>MKFPHDFLFGAASASYQVEGAWNEDGKGVTNWDEFSKIPGKTYNGTNGDIAVDHYHRYKEDVRLMAEMGLESYRFSISWARILPTGDGKVNEKGIEFYNNLIDECLKYGIVPFVTLYHWDLPLPLEKDGGWTNKRTAEAFVKYAETCFKAFGDRVKHWITFNETVMFCGLGYLKGAHPPGIQNDVPKYFQATHYVFYAHAKTVAVYKQLKQYGEIGITHVFLPAYSVDDQKENIQAANHANEYETYWYYDPILKGEYPSYVVQQLKEKGWTPNWTVEELEIIKQNAEENDFIGLNYYQPIRVERYDMDIKSEEHSRENSTLAPGNPSFDGFYRTVKMDDKTYTKWGWEISPEGFLEGLHMLKARYGDIKMYVTENGLGDEDPIIDGEIVDVPRIKFIEAHLKVMKRAIEEGINLKGYYAWSVIDLLSWLNGYKKQYGFIFVDHNDNLKRKKKLSFHWYKRVVETRGEELHHHHHH[2x]

In summary, we have characterized a novel PvGal-ase encoded by ORF1119 in Bacillus strain HMA207. The overall structure of ORF1119 was similar to those of other GH1 enzymes, which have a typical (β/α)8 barrel fold. The active site is located at the bottom of the pocket formed by loops of the barrel, a characteristic of most GH1 enzymes. The catalytic nucleophile (E374) and the catalytic acid/base (E163) residues of ORF1119 were conserved with other GH1 enzymes.

Structures of the ligand-free form and PvGal-bound form were determined at 2.5 Å and 2.45 Å resolution, respectively. The crystals belonged to space group P3221 and contained two protein molecules in the asymmetric unit. Because the structures of all four chains (chains A and B in both the ligand-free and complex forms) were almost the same (root mean square deviation for Cα atoms, <0.6 Å), below we describe chain A of the PvGal-bound form.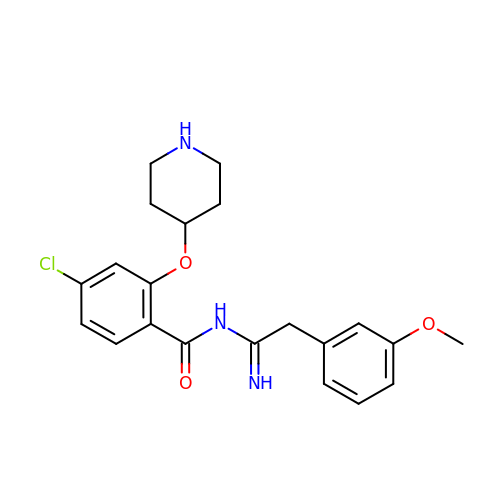4-chloranyl-N-[2-(3-methoxyphenyl)ethanimidoyl]-2-piperidin-4-yloxy-benzamide | C21 H24 Cl N3 O3 | LWKDHLRBDHZTMF-UHFFFAOYSA-N> MDEQVIFTTNTSGTIASVHSFEQINLRQCSTQSRNSCVQVGNKYLFIAQAQKALINVYNLSGSFKRESVEQRLPLPEILKCLEVVENDGVQYDRIQGVNHNLPDFNLPYLLLGSTESGKLYIWELNSGILLNVKPMAHYQSITKIKSILNGKYIITSGNDSRVIIWQTVDLVSASNDDPKPLCILHDHTLPVTDFQVSSSQGKFLSCTDTKLFTVSQDATIRCYDLSLIGSKKKQKANENDVSIGKTPVLLATFTTPYSIKSIVLDPADRACYIGTAEGCFSLNLFYKLKGNAIVNLLQSAGVNTVQKGRVFSLVQRNSLTGGENEDLDALYAMGQLVCENVLNSNVSCLEISMDGTLLLIGDTEGKVSIAEIYSKQIIRTIQTLTTSQDSVGEVTNLLTNPYRLERGNLLFEGESKGKQPSNNNGHNFMKIPNLQRVIFDGKNKGHLHDIWYQIGEPEAETDPNLALPLNDFNAYLEQVKTQESIFSHIGKVSSNVKVIDNKIDATSSLDSNAAKDEEITELKTNIEALTHAYKEL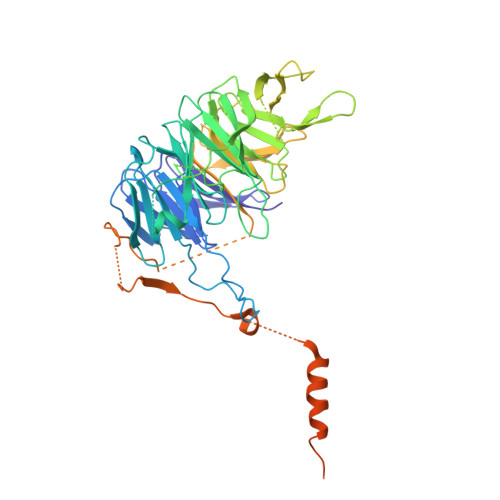RDMHEKLYEEHQQMLDKQ>[4x]SMQEKDASSQGFLPHFQHFATQAIHVGQDPE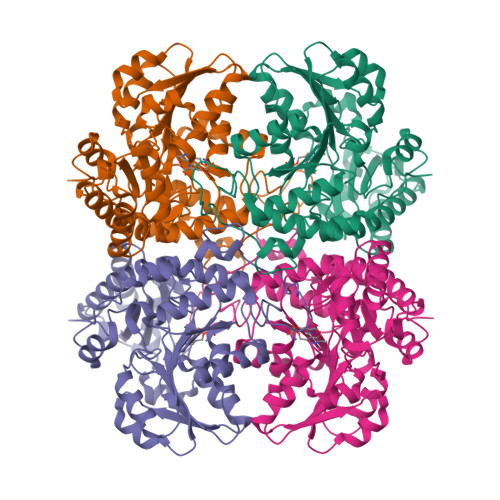QWTSRAVVPPISLSTTFKQGAPGQHSGFEYSRSGNPTRNCLEKAVAALDGAKYCLAFASGLAATVTITHLLKAGDQIICMDDVYGGTNRYFRQVASEFGLKISFVDCSKIKLLEAAITPETKLVWIETPTNPTQKVIDIEGCAHIVHKHGDIILVVDNTFMSPYFQRPLALGADISMYSATKYMNGHSDVVMGLVSVNCESLHNRLRFLQNSLGAVPSPIDCYLCNRGLKTLHVRMEKHFKNGMAVAQFLESNPWVEKVIYPGLPSHPQHELVKRQCTGCTGMVTFYIKGTLQHAEIFLKNLKLFTLAESLGGFESLAELPAIMTHASVLKNDRDVLGISDTLIRLSVGLEDEEDLLEDLDQALKAAHPPSG>[2x]GSQEGKKGKTTIKTGASVLNKWQMNPYDRGSAFAIGSDGLCCQSREVKEWHGCRATKGLMKGKHYYEVSCHDQGLCRVGWSTMQASLDLGT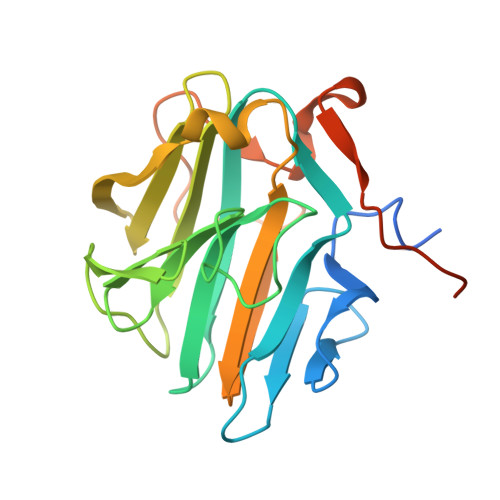DKFGFGFGGTGKKSHNKQFDNYGEEFTMHDTIGCYLDIDKGHVKFSKNGKDLGLAFEIPPHMKNQALFPACVLKNAELKFNFGEEEFKFPPKDGFVALSKAPDGYIVKSQHSGNAQVTQTKFLEHHHHHH>[6x]MDKTHVLRNTTRGMFRTSMMRVLGRPGSLSVTASAGGTACVPMAALLRRSATPAAASATAASAMSALWCTRCFESSSAGSPPKVSDAGMKERSTQEPCVAATPTPSDTAATLAAAATPAPAAPIKSKGVDYARLYAHHPIDYER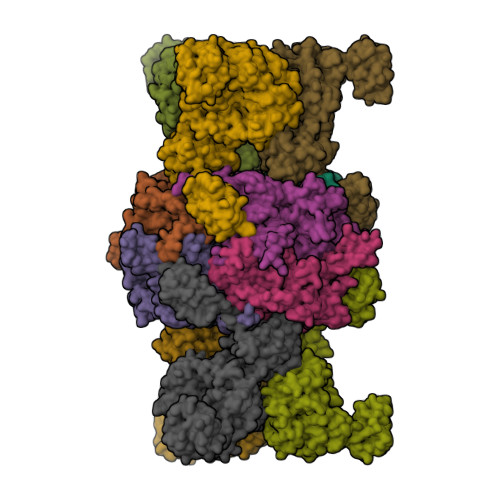STSKSPNILRLPANTSDPTYQENMARMEGLVEQLRARVRYVQAGGVVPEEEAAKAGVSISSIEADDRVRKLHLSRGKMLARDRIERLIDPGTRFLELSQLAGWDLYWDDKKKEYERCYSGGIVTGIGLVNGVRCMLVANDATVKGGTYYPITVKKHLRAQKIAEQNHLPCIYLVDSGGANLSRQDDVFPDEQHFGRIFYNEAQMSIKSISQIAVVMGSCTAGGAYVPAMADENIIVARNGTIFLGGPPLVLAATGEKVSSEELGGADVHCRISGVGDHYATDDLHALYLARRAVANLNLKEHNEARNPTDVKPVPPLYDPRELGGFIPDMLSDVVKSFDVRAIIARIVDGSRFDEFKALYGNTLVCGFARIEGMQVGIIANQGILYSESALKGAHFIGLCTQRNVPLLFLQNITGFMVGKKYEEGGIARNGARLVMAVSSAPVPKVTVLIGGSYGAGNYGMCGRAFEPRFLFMWPNARISVMGGTQAATVLTLTNRNLKNASEAEIAAFKDKVKKKYEKEGSCYYSTARLWDDGVIAPEDTRVVVAEALRATRLAPMEKRERV;>MLRYTGLWRERKVEKLLVANRGEIACRVFRTCREMHIRTVALFCEAERNAKHVAEADEAVCIGPPPAVNSYLRGEHIISVAKQLNVDAIHPGYGFLSENASFADAITRSGIEFIGPPASAISLMGSKSESKRIMEAAGVPVVPGYYGENQNVSFLAEEAKKVGFPILIKAVSGGGGKGMKIVERPEDFTFMLESAKREATNFFKDDRVILERYVKRSRHIECQIFFDKHGRGVFFFERDCSVQRRYQKVLEEAPAPHLSMETRQRIGEVALQAAKAVGYVGAGTVEFIFDTSTGEFYFMEMNTRLQVEHPVTEEVCRIKGAPLDLVKLQIKTAMGKPLTFSQEDVTLVGSCIEARVYAESPERGFLPESGPLTFIREPFQGVRGPARTRLDTGFREGDNVLIHYDPMLAKVISWGRSREEALRGLRQALGEYKVAGINTNIEFLKRCCETPEFARGGVTTNFISEHESQLLKSPVVTPEVAAMAATAWLLNRCDNWRGAFRLNSDTNATVHFYIDDHPVEVRLHTEGANYHKIFFSVWDHDGSFEVCSGPVTSKHRDQKSIVNDFTFLFENGMHHTVLAVATEGDVTVIGSFGLHQLRLLPLTDGFGDSSTAGGTSTKIVSPMPGKVSKLLVKSGDLVEKGQVLVIVEAMKMEHPVRALQDGRVSFLVKEGEVVGGDHVLATVAEEE[6x]3-SULFOPROPANOIC ACID | C3 H6 O5 S | 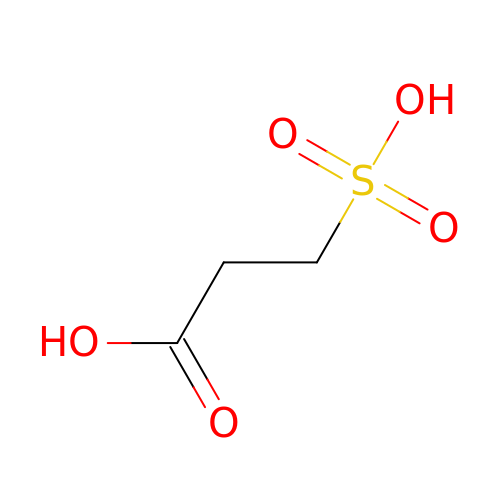OURSFPZPOXNNKX-UHFFFAOYSA-N>[4x]MSKATYKERAATHPSPVAAKLFNIMHEKQTNLCASLDVRTTKELLELVEALGPKICLLKTHVDILTDFSMEGTVKPLKALSAKYNFLLFEDRKFADIGNTVKLQYSAGVYRIAEWADITNAHGVVGPGIVSGLKQAAEEVTKEPRGLLMLAELSCKGSLATGEYTKGTVD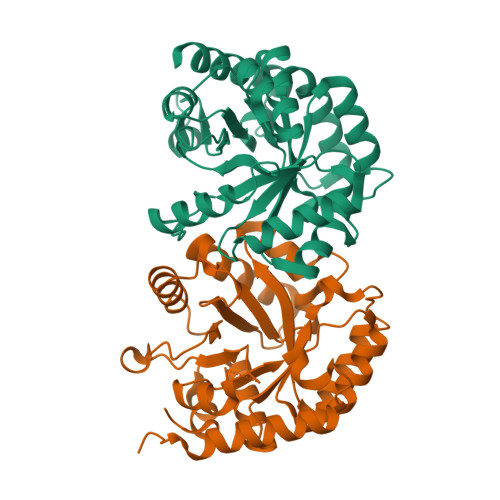IAKSDKDFVIGFIAQRDMGGRDEGYDWLIMTPGVGLDDKGDALGQQYRTVDDVVSTGSDIIIVGRGLFAKGRDAKVEGERYRKAGWEAYLRRCGQQN>MSEDIRRGPGRPPKKRVVPNFERKGILEKPVRPQSRLEFSYDNPLIFKNLFIYFKNLKSKNILVRCTPTEITFFSRDQSQASFVIATIDGKNVNHYYASDVFWLGINRELVEKMFNSIDRSFLKITIVHRYDKPETLFFIFTDFDIDKECTYQITVSEPELDMDLIEMEKSISEERLKNYPLRWEFTSKQLKKTFSDLSNYTELVTIEKLGGDTPLHLYFQKFNSISYHEMYKSSNKINLTSTIPKSQVFQINVKI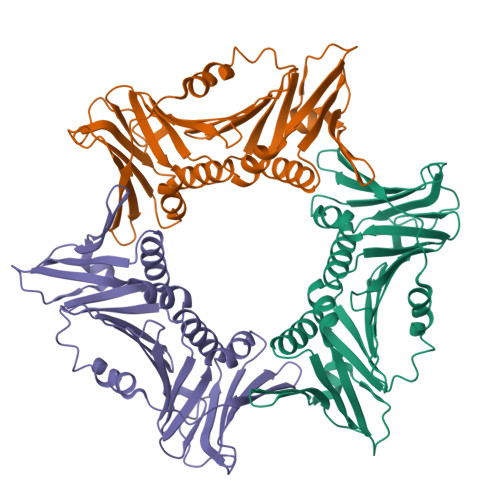AHIKSLASAMVTDKIRILCEENGNLIFQSEMDALMLNTITLNNTIGSSSHHHHHH[2x]L-glucono-1,5-lactone 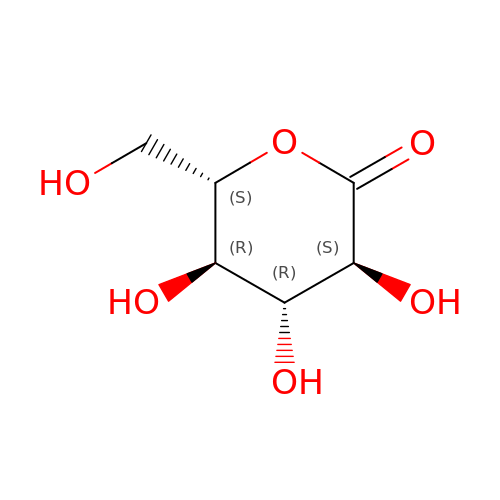| C6 H10 O6 | PHOQVHQSTUBQQK-KLVWXMOXSA-N> MDDLDALLA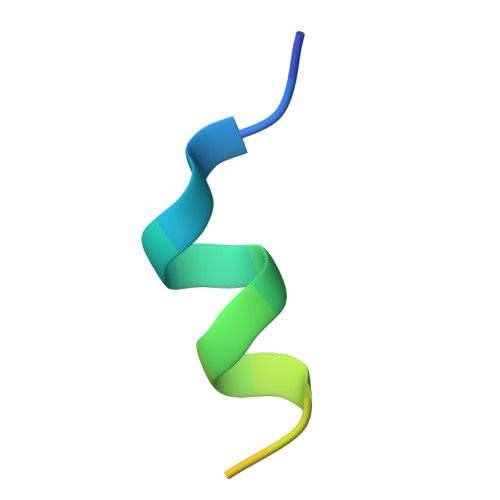DLESTTSHISK>HMSVILDTKGEPVSNAADAYYLVPVSHGEGGLALAKVGNEAEPKAVVLDPHHRPGLTVRFETPLAIAIITESFFLNIKFVPSSSDSEVWDVSKQYPIGLAVKVTDTKSFVGPFRVEK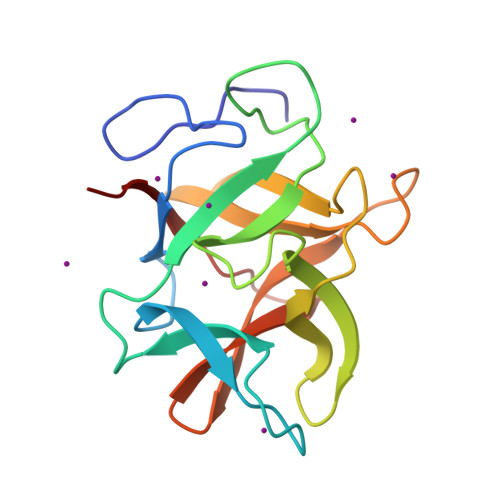EGEGYKIVYYPDRGQTGLDIGLVHRNDKYYLAATEGEPFVFKIRKATYE[2x]The pathway preference appears to depend on nitrogen availability, being the ornithine route preferred under nitrogen-rich conditions. Both routes converge at the generation of P5C, which in the final step is reduced to L-proline by P5C reductase (P5CR, EC 1.5.1.2). Here we report the high-resolution crystal structure of P5CR from M. truncatula (Mt), a model legume plant. The donut-shaped decamer of MtP5CR can be described as a pentamer of symmetric, bean-like dimers that are related to each other by a five-fold NCS axis. The catalytic centers of P5CRs are located between the dinucleotide-binding domain (N-terminal) and the dimerization domain (C-terminal).

In this paper, the term “unliganded” refers to the structure without a coenzyme or L-proline, despite the fact that it actually contains non-protein and non-solvent ligands. In apo structures (unliganded and complexed with L-proline) loop L3 occupies a part of the coenzyme-binding site. Moreover, in these two complexes the imidazole ring of His45 lies in a structural position similar to that of adenine from NAD(P)+. On the contrary, in the crystal structures of unliganded MtP5CR and both holo complexes, chloride anions are present in the catalytic center. Also, highly positive peaks in Fo–Fc electron density maps appear if a water molecule is placed instead of the chloride, suggesting a larger atom. The presence of chlorides was verified with the use of anomalous difference electron density map, resulting from diffraction data collected at 1.7196 Å wavelength. In the crystal structures of unliganded MtP5CR and both holo-complexes, chloride anions were found in the catalytic centers at the same structural positions as the carboxyl groups of L-prolines in the MtP5CR/L-proline complex. Therefore, as inferred from the crystal structures, chloride ions should be rather inhibitory as they compete for the same site with the carboxylic group of L-proline and, most probably, P5C. Indeed, the concentration of Cl− ions in the crystallization drop when the crystals were harvested should have exceeded 340 mM. As a consequence, we propose that the Cl− found in the crystal structure reflects the inhibitory role of Cl−.

>[10x]SNAMEIIPIPADSYTLGFIGAGKMAESIAKGAVRSGVLSPSRIKTAIHSNPARRTAFESIGITVLSSNDDVVRDSNVVVFSVKPQLLKDVVLKLKPLLTKDKLLVSVAAGIKMKDLQEWAGHERFIRVMPNTAATVGEAASVMSLGGAATEEDANLISQLFGSIGKIWKADDKYFDAITGLSGSGPAYIYLAIEALADGGVAAGLPRDLALSLASQTVLGAASMATQSGKHPGQLKDDVTSPGGTTIAGVHELEKAGFRGILMNAVVAAAKRSQELS>[4x]KIEAVIFDWAGTTVDYGCFAPLEVFMEIFHKRGVAITAEEARKPMGLLKIDHVRALTEMPRIASEWNRVFRQLPTEADIQEMYEEFEEILFAILPRYASPINAVKEVIASLRERGIKIGSTTGYTREMMDIVAKEAALQGYKPDFLVTPDDVPAGRPYPWMCYKNAMELGVYPMNHMIKVGDTVSDMKEGRNAGMWTVGVILGSSELGLTEEEVENMDSVELREKIEVVRNRFVE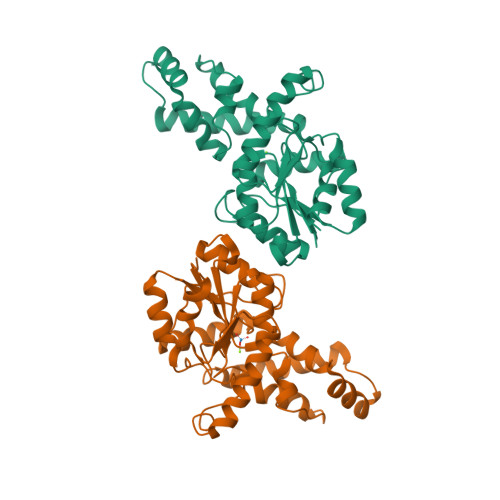NGAHFTIETMQELESVMEHIE>MSLLSKTRELNTLLQKHKGIAVDFKDVAQTISSVTVTNVFIVSRRGKILGSSLNELLKSQRIIQMLEERHIPSEYTERLMEVKQTESNIDIDNVLTVFPPENRELFIDSRTTIFPILGGGERLGTLVLGRVHDDFNENDLVLGEYAATVIGMEILREKHSEVEKEARDKAAITMAINSLSYSEKEAIEHIFEELGGTEGLLIASKVADRVGITRSVIVNALRKLESAGVIESRSLGMKGTFIKVKKEKFLDELEKS[2x]

In Gram-positive pathogens such as Staphylococcus aureus (Sa) and Enterococcus faecalis (Ef), the pleiotropic transcription factor CodY plays a key role in integrating metabolism and virulence factor expression. CodY DNA-binding is activated by two types of ligands: branched chain amino acids (BCAAs, i.e. isoleucine, leucine, and valine) and, in most cases, guanosine triphosphate, GTP. Each 30 kDa protomer comprises the N-terminal ligand-binding domain called GAF (cGMP-specific phosphodiesterases, adenylyl cyclases and FhlA). The GAF domain is connected by an extended linker helix to the C-terminal DNA-binding (DBD) domain that contains a winged helix-turn-helix (wHTH) motif.

The crystal structure of the SaCodY–DNA complex—also presented below—had Ile/GTP-bound GAF domains. The SaCodY-DNA complex was co-crystallized with Ile and GTP. The Ile/GTP-bound GAF domains of SaCodY in its free and DNA-bound forms are essentially identical, demonstrating that the GAF domains do not undergo a structural change upon DBD domain-DNA interaction. In the crystals, two CodY dimers bind to a single DNA duplex. The dimers are related by a 60° rotation and a 30-Å translation along the DNA, binding one side of the DNA helix. The spatial relationship of the two dimers of SaCodY is defined by a crystallographic axis. DNA interactions are primarily mediated by hydrogen bonds of residues with the sugar–phosphate backbone of the DNA, indicative of an indirect or shape readout mechanism. What follows is a detailed description of the interactions between protomer B of SaCodY and the 5′ half-site DNA. The position of the recognition helix in the major groove is stabilized by hydrogen bonds of recognition helix residues Thr213 and Arg222 to backbone phosphates of T5, T6 and T17’ located on opposite sides of the major groove (the prime-sign indicates template strand nt). Ser215, located at the recognition helix N-terminus, forms the only base-specific hydrogen bond between the recognition helix and major groove bases.>[2x]GPHMAALRPRLVFHTQLAHGSPTGRIEGFTNVKELYGKIAEAFRLPAAEVMFCTLNTHKVDMDKLLGGQIGLEDFIFAHVKGQRKEVEVFKSEEALGLTITDNGAGYAFIKRIKEGSVIDHIQLISVGDMIEAINGQSLLGCRHYEVARLLKELPRGRTFTLKLTEPRKAFDMISQRSAGGHPGSGPQLGTGRGTLRLRSRGPATVEDLPSAFE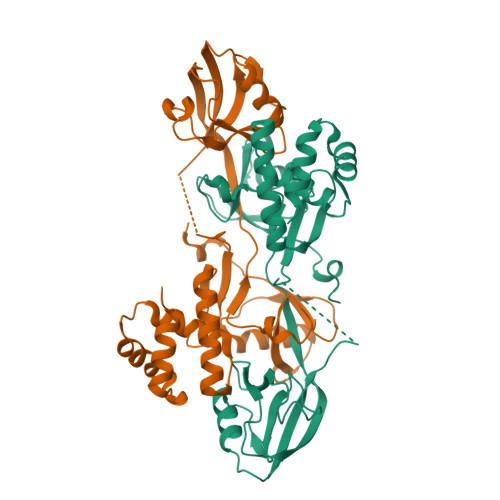EKAIEKVDDLLESYMGIRDTELAATMVELGKDKRNPDELAEALDERLGDFAFPDEFVFDVWGAIGD DNA gyrase, a bacterial type II topoisomerase, is a clinically validated antibacterial target. Unlike most bacterial species that have both DNA gyrase and topoisomerase IV (topoIV), M. tuberculosis has only the DNA gyrase enzyme, but with a simultaneous functional role of topoIV. It performs the essential function of introducing negative supercoils into the DNA as well as decatenation activity. Structurally, DNA gyrase is a heterotetrametric enzyme with two GyrA and two GyrB subunits (A2B2).

Here, we present the first 2.8 Å resolution crystal structure of compound 5 in complex with the M. tuberculosis DNA gyrase core fusion and a DNA fragment. The LHS (methoxy-naphthyridine) moiety of compound 5 intercalates between the DNA base pairs along the 2-fold axis of the complex, positioned midway between the two DNA cleavage sites. Additionally, the 3,5-difluoro-4-bromo phenyl RHS moiety occupies a deep, hydrophobic binding pocket formed at the interface of both GyrA subunits in a similar fashion as our previously disclosed cocrystallized NBTI AMK-12 in a complex with S. aureus DNA gyrase. Moreover, this crystal structure once again revealed that the asymmetry of 5 (with respect to the LHS moiety) induces the asymmetry in the nicked DNA conformation, which in turn affects the configuration of the catalytic site. The compound 5 was present in the crystal structure as a racemic mixture, since the two enantiomers were not separated prior to the crystallization experiment, and each stereoisomer was modeled with a 50% occupancy. The 3,5-difluoro-4-bromo phenyl RHS moiety is tightly embraced by the surrounding amino acid residues in a tight pocket between the two GyrA subunits. This pocket is predominantly hydrophobic and consists of the amino acids Ala74, Ala78, Met81, and Met127, engaged primarily in van der Waals interactions with the RHS moiety. The crystal structure reveals another feature of RHS binding, namely, the halogen bonding interaction between the bromine and the backbone carbonyl oxygens of both GyrA Ala74 residues, which provides a symmetric binding site. Both stereoisomers form bifurcated halogen bonds, with one forming fully symmetrical halogen bonds and the other forming less symmetrical halogen bonds. The secondary linker of 5 forms a salt bridge with the carboxylate of Asp89. Another feature that emerges from the present crystal structure is that the hydroxyl group in the linker in 5 can form a hydrogen bond with an adenine as a DNA base (distance: 2.8 Å, angles: 126.5° and 115.2°).

>SNALVRRKSATDIGGLPGKLADCRSTDPRKSELYVVEGDSAGGSAKSGRDSMFQAILPLRGKIINVEKARIDRVLKNTEVQAIITALGTGIHDEFDIGKLRYHKIVLMADADVDGQHISTLLLTLLFRFMRPLIENGHVFLAQPPLYKLKWQRSDPEFAYSDRERDGLLEAGLKAGKKINKEDGIQRYKGLGEMDAKELWETTMDPSVRVLRQVTLDDAAAADELFSILMGEDVDARRSFITRNAKDVRFLDVTDTTLPPDDSLDRIEPVDIEQEMQRSYIDYAMSVIVGRALPEVRDGLKPVHRRVLYAMFDSGFRPDRSHAKSARSVAETMGNYHPHGDASIYDSLVRMAQPWSLRYPLVDGQGNFGSPGNDPPAAMRYTEARLTPLAMEMLREIDEETVDFIPNYDGRVQEPTVLPSRFPNLLANGSGGIAVGMATNIPPHNLRELADAVFWALENHDADEEETLAAVMGRVKGPDFPTAGLIVGSQGTADAYKTGRGSIRMRGVVEVEEDSRGRTSLVITELPYQVNHDNFITSIAEQVRDGKLAGISNIEDQSSDRVGLRIVIEIKRDAVAKVVINNLYKHTQLQTSFGANMLAIVDGVPRTLRLDQLIRYYVDHQLDVIVRRTTYRLRKANERAHILRGLVKALDALDEVIALIRASETVDIARAGLIELLDIDEIQAQAILDMQLRRLAALERQRIIDDLAKIEAEIADLEDILAKPERQRGIVRDELAEIVDRHGDDRRTRIIAIGSG[2x]> GSMTSPRNCLR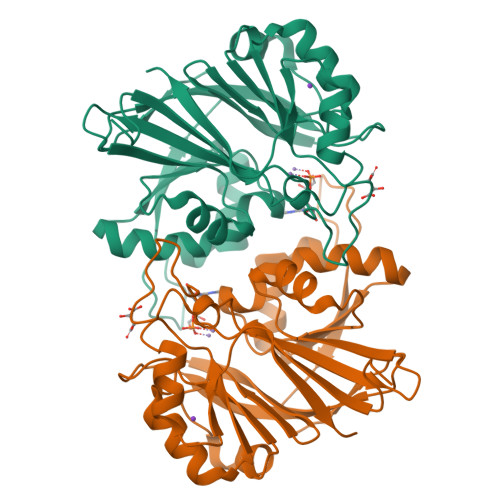FTLLGCGSSPGVPRINGDWGKCDPKNPKNRRRRASLLVERYDAEGNNTVVVIDTGPDFRMQMIDSGVHMLDAAVYTHPHADHIHGIDDLRTYVVDNGRLMDVYANRLTRNRLYDTFGYCFETPVGSSYPPILSMHDIAPETPFSIEGAGGAIRFEPFSQVHGDIESLGFRIGSVVYCTDVSAFPEQSLQYIKDADVLIIGALQYRPHPSHFSLGEALEWIEKLSPKRAILTHMHVPLDYETVMRETPHHVEPGYDGLRFEVAV>[10x]MFFSRLSLSALKAAPAREALPGLLSRQSFSSAGFSQFSSQKFFFSPSRNFSQSPLFQKHTPVHCNQRIASALVPTQQPAMTRQNPYAMQVGARYDAGVASLSAAIALMSVGGVAQGIGSLFAALVSGTARNPSIKEDLFTYTLIGMGFLEFLGIICVLMSAVLLYS;> MAAGSRFPFCTAARLSSRGTLPRLGEATFFAGAESQRSAGAFAKTLQRPFLRAPSTQLFPVGNRLGVSSARALVANAMEPRRFFAAAASAKATHALQPTGTGSVAFTRPGQGSNAQFQTSLADKTRGLLGVGFLRPTKMASFAATFLLNFRFYFMYMARTTFQAVRPLLAFSVFGEVMKLVLATMSSGLFSFLFSFVLAFEVFYFFLQCYISYTFLTMFFTVLF;> MVRNQRYPASPVQEIFLPEPVPFVQFDQTAPSPNSPPAPLPSPSLSQCEEQKDRYRDISSMFHRGVAGAEQVREAYNSMAKCFRRVSVAEVLESDPAFRQARNFTMDLKQAEDDQRYKQLQYGRVPSILTKYHL;> MFARAFSRFASLAAPAPQRGWNAFVLPSRHFATAAGGANPFKNQLLLTLSSPSEAIYVRTPVRSVTVPGSEGAMTMTNGHSQTVARLKAGEIIVRKGETGDEVERFFLSDGFVLFKSPEDDSGCCTAEVLGVEVVPVSMLDKESAATALQELLQQGAGATDEWTKARTLLGQELLSSVIRAAP;> MWRSSGVSFTRYASEMAALLRQCLKEPYRTQAMQRNQIHLKETVYQQGQVLTRETFNDIKKAFEAAAKHAGEK;> MAGLASLSSVGALRGMRLVPAAHLLPLHSAFGQQTRNFGAGDLKIVAARMKSVKSIQKITKAMKMVAASKLRMDQRRLENGLPFATPVQKLVQRIPVDPKEKGTLAVLALSSDKGLCGGVNSFVAKQARIVIKENEMAGNAVQVYGVGDKIRSALQRTFGDRFKRIMTE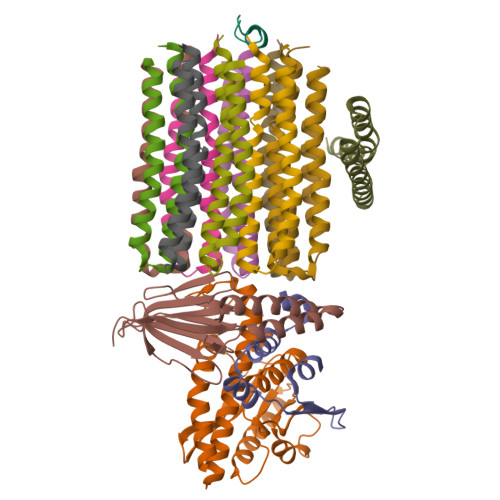VTRFPWNFGQACIIADRLMQDNPARLMVIYNHFKSAVAYDTLTLNVLTPTQAAQSAKEQLNTFEFEPEKTDVWKDLQDFYYACTVFGCMLDNIASEQSARMSAMDNASTNAGEMISSLTLRYNRARQAKITTELVEIISGANALE>[3x]MGSGLNKFIYVGLVISQLLTLAAYVVVTAGAALLQKKANTLTLFDTQEGIDKYTPVYKEVFTATTYIIAYPQQPQYQFQYQWWIIQFELFVFLLTAACTVFPSIIKRMRP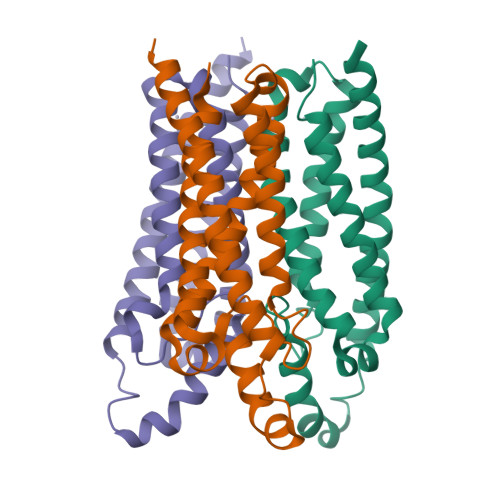VALTFIASALVLVMDNINAIFFLLRNETAKAVFDDYRIATAQAGLIMVGVANGLTIFFLGSYDAEESHAMPNVHVTSDGATKVSNSLVPR(3~{S},6~{S})-3-(1~{H}-imidazol-4-ylmethyl)-6-propan-2-yl-piperazine-2,5-dione 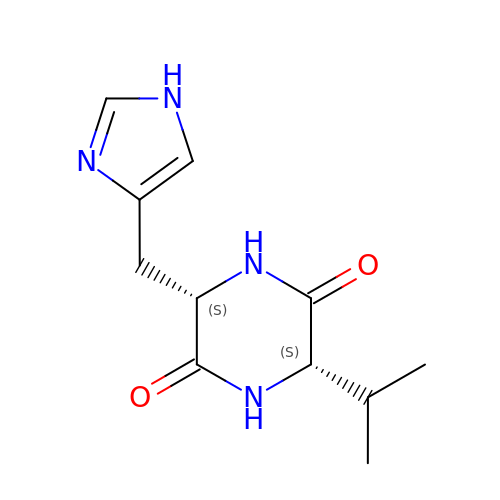| C11 H16 N4 O2 | CNEIXWVYFRHWEJ-IUCAKERBSA-N>HHHH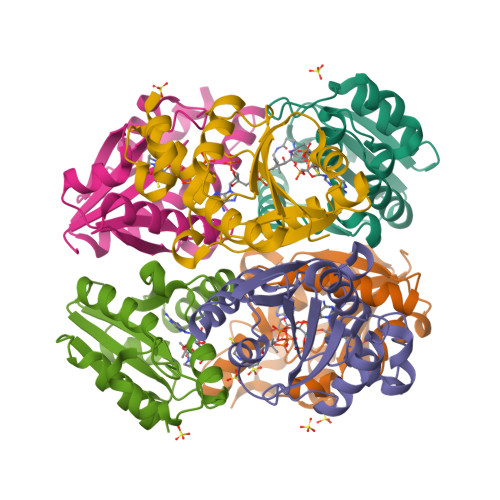HHMQKIGIYPGTFDPVTNGHIDIIHRSSELFEKLIVAVAHSSAKNPMFSLDERLKMIQLATKSFKNVECVAFEGLLANLAKEYHCKVLVRGLRVVSDFEYELQMGYANKSLNHELETLYFMPTLQNAFISSSIVRSIIAHKGDASHLVPKEIYPLISKA[6x]> GDRVADVIESSIGDSVSRALTQALPAPTGQNTQV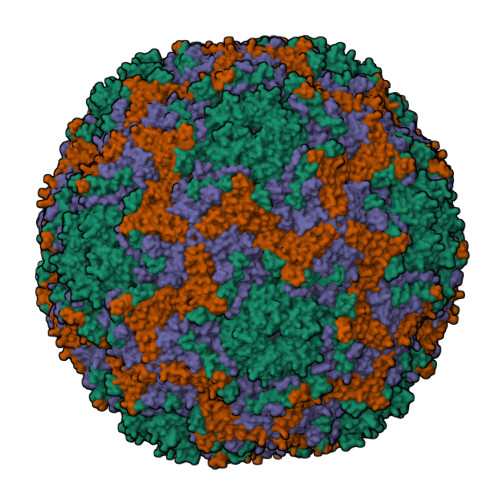SSHRLDTGEVPALQAAEIGASSNTSDESMIETRCVLNSHSTAETTLDSFFSRAGLVGEIDLPLEGTTNPNGYANWDIDITGYAQMRRKVELFTYMRFDAEFTFVACTPTGQVVPQLLQYMFVPPGAPKPESRESLAWQTATNPSVFVKLTDPPAQVSVPFMSPASAYQWFYDGYPTFGEHKQEKDLEYGACPNNMMGTFSVRNVGSSKSKYPLVVRIYMRMKHVRAWIPRPMRNQNYLFKANPNYAGNSIKPTGTSRTAITTL;> SPSAEACGYSDRVAQLTIGNSTITTQEAANIIVGYGEWPSYCSDDDATAVDKPTRPDVSVNRFYTLDTKLWEKSSKGWYWKFPDVLTETGVFGQNAQFHYLYRSGFCIHVQCNASKFHQGALLVAILPEYVIGTVAGGTGTEDSHPPYKQTQPGADGFELQHPYVLDAGIPISQLTVCPHQWINLRTNNCATIIVPYMNTLPFDSALNHCNFGLLVVPISPLDFDQGATPVIPITITLAPMCSEFAGLRQAVTQ;> GFPTEPKPGTNQFLTTDDGVSAPILPNFHPTPCIHIPGEVRNLLELCQVETILEVNNVPTNATSLMERLRFPVSAQAGKGELCAVFRADPGRDGPWQSTMLGQLCGYYTQWSGSLEVTFMFTGSFMATGKMLIAYTPPGGPLPKDRATAMLGTHVIWDFGLQSSVTLVIPWISNTHYRAHARDGVFDYYTTGLVSIWYQTNYVVPIGAPNTAYIIALAAAQKNFTMKLCKDTSHILQTASIQ;> MGSQVSTQRSGSHENSNSATEGSTINYTTINYYKDSYAATAGKQSLKQDPDKFANPVKDIFTEMAAPLK> MLSHMVLTRQDIGRAASYYEDGA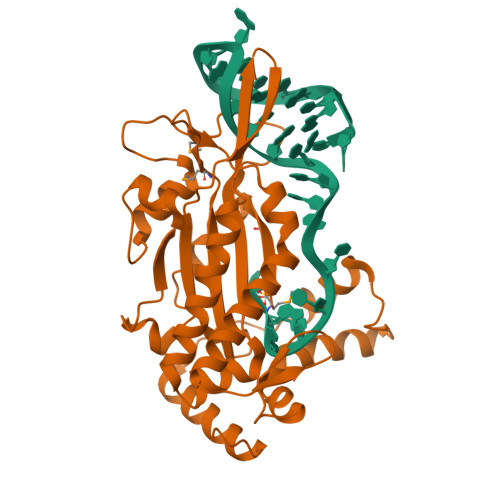DDYYAKDGDASEWQGKGAEELGLSGEVDSKRFRELLAGNIGEGHRIMRSATRQDSKERIGLDLTFSAPKSVSLQALVAGDAEIIKAHDRAVARTLEQAEARAQARQKIQGKTRIETTGNLVIGKFRHETSRERDPQLHTHAVILNMTKRSDGQWRALKNDEIVKATRYLGAVYNAELAHELQKLGYQLRYGKDGNFDLAHIDRQQIEGFSKRTEQIAEWYAARGLDPNSVSLEQKQAAKVLSRAKKTSVDREALRAEWQATAKELGIDFS>MIPPPEKVRMNSVNFKNILQWEVPAFPKTQLTFTAQYESYRSFQDHCKRTASTQCDFSHLSKYGDYTVRVRAELADEHSEWVQVTFCPVEDTIIGPPEMQIESLAESLHLRFSAPQIENEPETWTLKNIYDSWAYRVQYWKQGTNEKFQVVSPYDSEVLRNLEPWTTYCIQVQGFLLDQQRTGEWSEPICERTGNDEITPSGGS[12x];>[12x]LLQHVKFQSSNFENILTWDGGPASTSDTVYSVEYKKYGERKWLAKAGCQRITQKFCDLTMETRDHQEFYYAKVTAVSAGGPPVTKMTDRFSSLQHTTIKPPDVTCIPKVRSIQMLVHPTLTPVLSEDGHQLTLEEIFHDLFYRLELHVNHTYQMHLEGKQREYEFLGLTPDTEFLG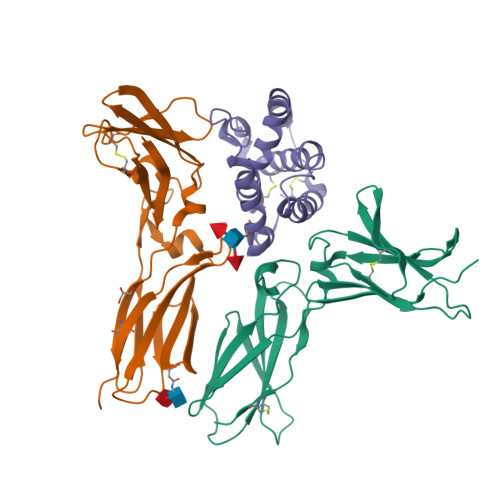SITILTPILSKESAPYVCRVKTLPDGGS;>LPVNTRCKLHVRNFQSPYIVNRTFMLAKEASLADQNTDVRLIGEKLFRGVSAKDQCYLMKQVLQFTLEDVLLPQSDRFQPYMWEVVPFLTKLSNKLSSCHISGDDQNIQKNVRRLKETVKKLGESGEIKAIGELDLLFMSLRNACVGGS[12x]>[2x]MRVNNGLTPQELEAYGISDVHDIVYNPSYDLLYQEELDPSLTGYERGVLTNLGAVAVDTGIFTGRSPKDKYIVRDDTTRDTFWWADKGKGKNDNKPLSPETWQHLKGLVTRQLSGKRLFVVDAFCGANPDTRLSVRFITEVAWQAHFVKNMFIRPSDEELAGFKPDFIVMNGAKCTNPQWKEQGLNSENFVAFNLTERMQLIGGTWYGGEMKKGMFSMMNYLLPLKGIASMHCSANVGEKGDVAVFFGLSGTGKTTLSTDPKRRLIGDDEHGWDDDGVFNFEGGCYAKTIKLSKEAEPEIYNAIRRDALLENVTVREDGTIDFDDGSKTENTRVSYPIYHIDNIVKPVSKAGHATKVIFLTADAFGVLPPVSRLTADQTQYHFLSGFTAKLAGTERGITEPTPTFSACFGAAFLSLHPTQYAEVLVKRMQAAGAQAYLVNTGWNGTGKRISIKDTRAIIDAILNGSLDNA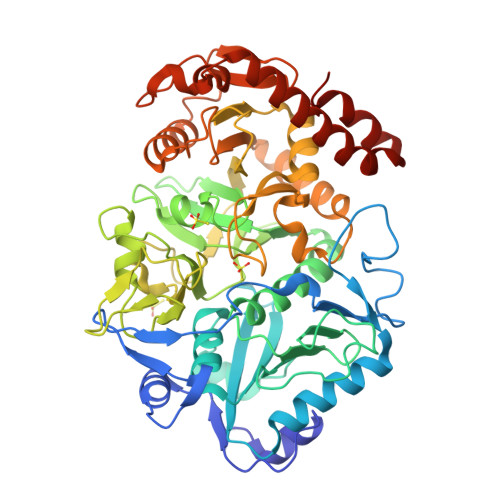ETFTLPMFNLAIPTELPGVDTKILDPRNTYASPEQWQEKAETLAKLFIDNFDKYTDTPAGAALVAAGPKLHHHHHH> RTDCYGNVNRIDTTGASCKTAKPEGLSYCGVSASKKIAERDLQAMDRYKTIIKKVGEKLCVEPAVIAGIISRESHAGKVLKNGWGDRGNGFGLMQVDKRSHKPQGT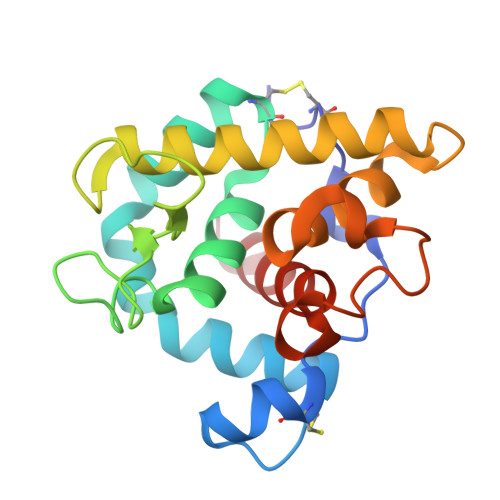WNGEVHITQGTTILINFIKTIQKKFPSWTKDQQLKGGISAYNAGAGNVRSYARMDIGTTHDDYANDVVARAQYYKQHGY> MGSQPTNSHFTLNEQTLCGTNISLLGNNRFIQIGNGLHMTYAPGFFGNWSRDLTIGPRFGGLNKQPIHVPPKRTETASIQVTPRSIVINRMNNIQINPTSIGNPQVTIRLPLNNFKSTTQLIQQVSLTDFFRPDIEHAGSIVLILRHPSDMIGEANTLTQAGRDPDVLLEGLRNLFNAC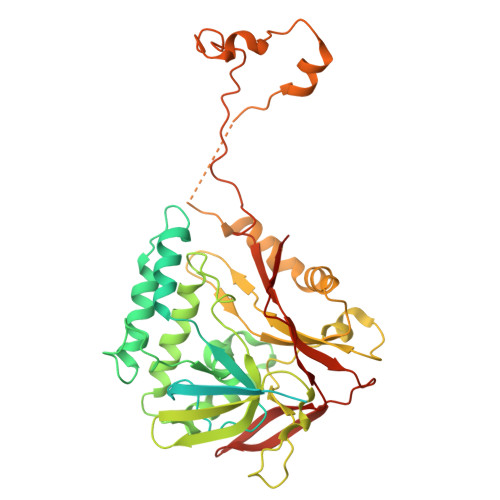TAPWTVGEGGGLRAYVTSLSFIAACRAEEYTDKQAADANRTAIVSAYGCSRMETRLIRFSECLRAMVQCHVFPHRFISFFGSLLEYTIQDNLCNITAVAKGPQEAARTDKTSTRRVTANIPACVFWDVDKDLHLSADGLKHVFLVFVYTQRRQREGVRLHLALSQLNEQCFGRGIGFLLGRIRAENAAWGTEGVANTHQPYNTRALPLVQLSNDPTSPRCSIGEITGVNWNLARQRLYQWTGDFRGLPTQLSCMYAAYTLIGTIPSESVRYTRRMERFGGYNVPTIWLEGVVWGGTNTWNECYY>VEYRNWSKPQCQITGFAPFSKDNSIRLSAGGDIWVTREPYVSCDPGKCYQFALGQGTTLDNKHSNDTVHDRIPHRTLLMNELGVPFHLGTRQVCIAWSSSSCHDGKAWLHVCITGDDKNATASFIYDGRLVDSIGSWSQNILRTQESECVCINGTCTVVMTDGSASGRADTRILFIEEGKIVHISPLSGSAQHIEECSCYPRYPGVRCICRDNWKGSNRPVVDINMEDYSIDSSYVCSGLVGDTPRNDDSSSNSNCRNPNNERG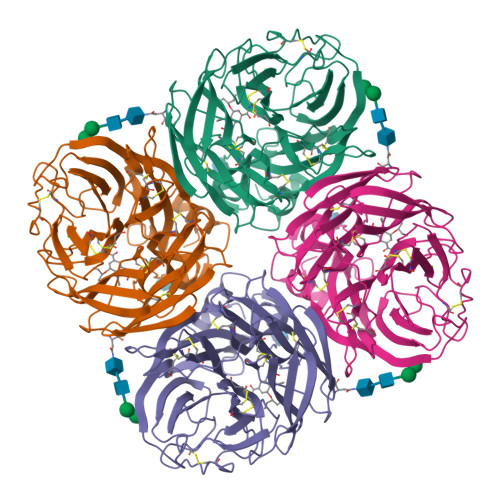TQGVKGWAFDNGNDLWMGRTISKESRSGYETFKVIGGWSTPNSKSQVNRQVIVDNNNWSGYSGIFSVEGKSCINRCFYVELIRGRPQETRVWWTSNSIVVFCGTSGTYGTGSWPDGANINFMPI[2x]17-{[ethyl(dihydroxy)-lambda~4~-sulfanyl]amino}-11,13-difluoro-2-methyl-6,7,8,9-tetrahydrodibenzo[4,5:7,8][1,6]dioxacyclododecino[3,2-c]pyridin-3(2H)-one 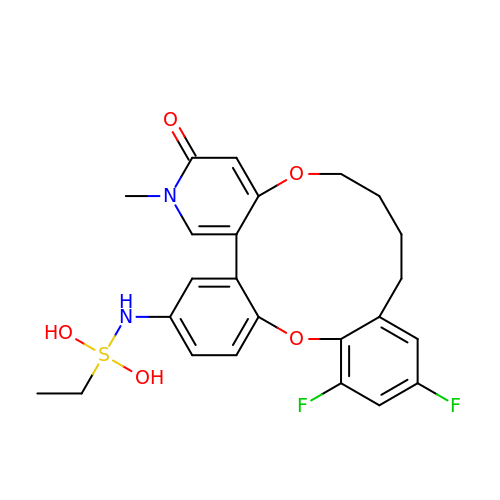| C24 H26 F2 N2 O5 S | VWDSFGMYIKNVLS-UHFFFAOYSA-N>MDDISQDNFLLSKEYENSLDVDTKKASGIYYTPKIIVDYIVKKTLKNHDIIKNPYPRILDISCGCGNFLLEVYDILYDLFEENIYELKKKYDENYWTVDNIHRHILNYCIYGADIDEKAISILKDSLTNKKVVNDLDESDIKINLFCCDSLKKKWRYKFDY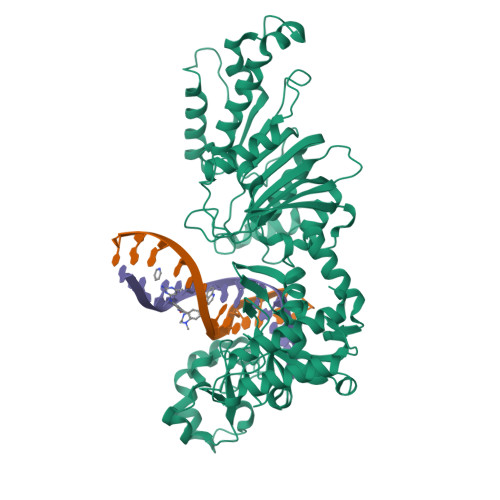IVGNPPYIGHKKLEKKYKKFLLEKYSEVYKDKADLYFCFYKKIIDILKQGGIGSVITPRYFLESLSGKDLREYIKSNVNVQEIVDFLGANIFKNIGVSSCILTFDKKKTKETYIDVFKIKNEDICINKFETLEELLKSSKFEHFNINQRLLSDEWILVNKDDETFYNKIQEKCKYSLEDIAISFQGIITGCDKAFILSKDDVKLNLVDDKFLKCWIKSKNINKYIVDKSEYRLIYSNDIDNENTNKRILDEIIGLYKTKLENRRECKSGIRKWYELQWGREKLFFERKKIMYPYKSNENRFAIDYDNNFSSADVYSFFIKEEYLDKFSYEYLVGILNSSVYDKYFKITAKKMSKNIYDYYPNKVMKIRIFRDNNYEEIENLSKQIISILLNKSIDKGKVEKLQIKMDNLIMDSLGI[3x]> MKGTIVGTWIKTLRD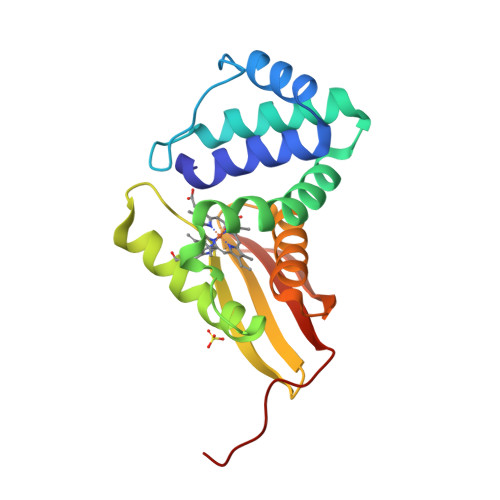LYGNDVVDESLKSVGWEPDRVITPLEDIDDDEVRRIFAKVSEKTGKNVNEIWREVGRQNFKTFSEWFPSYFAGRRLVNFLMMMDEVHLQLTKMIKGATPPRLIAKPVAKDAIEMEYVSKRKMYDYFLGFIEGSSKFFKEEISVEEVERGEKDGFSRLKVRIKFKNPVFEYKKN~{tert}-butyl 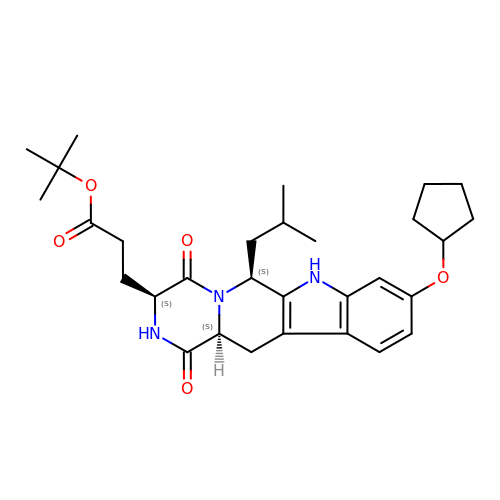3-[(2~{S},5~{S},8~{S})-14-cyclopentyloxy-2-(2-methylpropyl)-4,7-bis(oxidanylidene)-3,6,17-triazatetracyclo[8.7.0.0^{3,8}.0^{11,16}]heptadeca-1(10),11,13,15-tetraen-5-yl]propanoate | C30 H41 N3 O5 | MVNIRJAHJUCHLD-HVCNVCAESA-N> AFRYRREGQFTKFRVHFDRSGFRPYIDELKWEIMDWHYKRAMGPQMKKTLMSYQEGSEKLQYMHDLIALGTAKA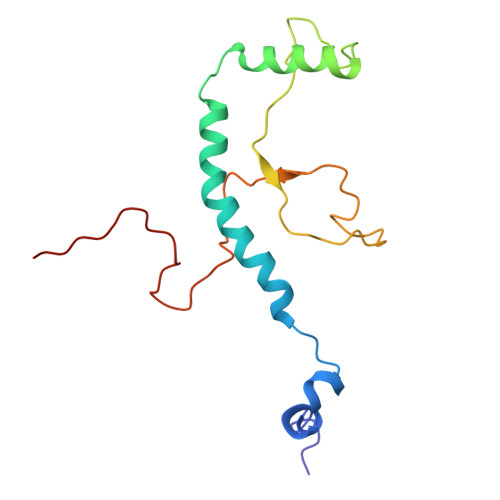KFPHATKRFFFVPALPVTIPYRRSSNPFCLLSANKTGWLQWSPKQRVPFPQPLGKRKVGGTDPQPPVFPK>MPFTIDSARGIFPNTLAADVVPATIARFSQLNAEDQLALIWFAYLEMGKTLTIAAPGAASMQLAENALKEIQAMGPLQQTQAMCDLANRADTPLCRTYASWSPNIKLGFWYRLGELMEQGFVAPIPAGYQLSANANAVLATIQGLESGQQITVLLNAVVDMGFTAGKDGKRIAEPVVPPQDTASRTKVSIEGVTNATVLNYMDNLNANDFDTLIELFTSDGALQPPFQRPIVGKENVLRFFREECQNLKLIPERGVTE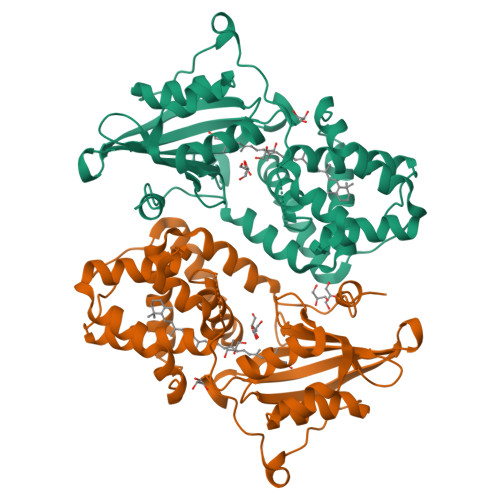PAEDGFTQIKVTGKVQTPWFGGNVGMNIAWRFLLNPEGKIFFVAIDLLASPKELLNFAVHHHHHH[2x]>SMVRRTKEEAQETRAQIIEAAERAFYKRGVARTTLADIAELAGVTRGAIYWHFNNKAELVQALLDSLHETHDHLARASESEDEVDPLGCMRKLLLQVFNELVLDARTRRINEILHHKCEFTDDMCEIRQQRQSAVLDIHKGWTLALANA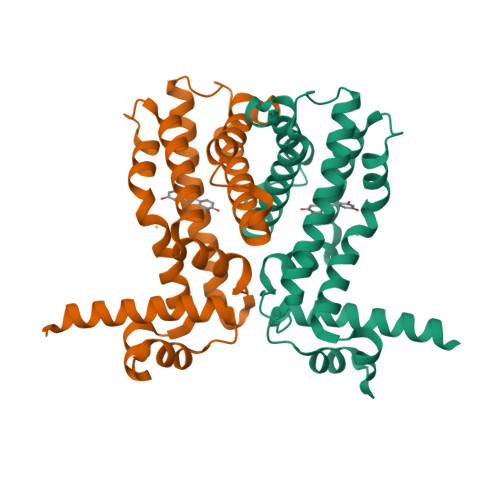VRRGQLPGELDAERAAVALYAYVDGLIRRWLLLPDSVDLLGDVEKWVDTGLDMLRLSPALRK[4x]>[6x]MGMQGDPDVLRLLNEQLT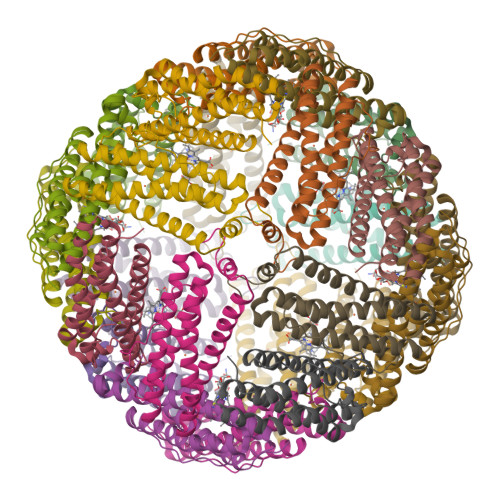SELTAINQYFLHSKMQDNWGFTELAAHTRAESFDEMRHAEEITDRILLLDGLPNYQRIGSLRIGQTLREQFEADLAIEYDVLNRLKPGIVMCREKQDTTSAVLLEKIVADEEEHIDYLETQLELMDKLGEELYSAQCVSRPPT>[6x]MIQGVIQKIAGPAVIAKGMLGARMYDICKVGEEGLVGEIIRLDGDTAFVQVYEDTSGLKVGEPVVSTGLPLAVELGPGMLNGIYDGIQRPLERIREKTGIYITRGVVVHALDREKKWAWTPMVKPGDEVRGGMVLGTVPEFGFTHKILVPPDVRGRVKEVKPAGEYTVEEPVVVLEDGTELKMYHTWPVRRARPVQRKLDPNTPFLTGMRILDVLFPVAMGGTAAIPGPFGSGKTVTQQSLAKWSNADVVVYVGCGERGNEMTDVLVEFPELTDPKTGGPLMHRTVLIANTSNMPVAAREASIYVGVTIAEYFRDQGFSVALMADSTSRWAEALREISSRLEEMPAEEGYPPYLAARLAAFYERAGKVITLGGEEGAVTIVGAVSPPGGDMSEPVTQSTLRIVGAFWRLDASLAFRRHFPAINWNGSYSLFTSALDPWYRENVAEDYPELRDAISELLQREAGLQEIVQLVGPDALQDAERLVIEVGRIIREDFLQQNAYHEVDAYCSMKKAYGIMKMILAFYKEAEAAIKRGVSIDEILQLPVLERIGRARYVSEEEFPAYFEEAMKEIQGAFKALA;>[6x]MDLLKKEYTGITYISGPLLFVENAKDLA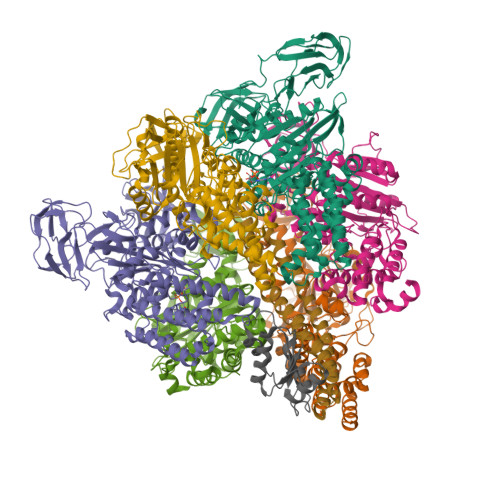YGAIVDIKDGTGRVRGGQVIEVSEEYAVIQVFEETTGLDLATTSVSLVEDVARLGVSKEMLGRRFNGIGKPIDGLPPITPEKRLPITGLPLNPVARRKPEQFIQTGISTIDVMNTLVRGQKLPIFSGSGLPANEIAAQIARQATVRPDLSGEGEKEEPFAVVFAAMGITQRELSYFIQEFERTGALSRSVLFLNKADDPTIERILTPRMALTVAEYLAFEHDYHVLVILTDMTNYCEALREIGAAREEIPGRRGYPGYMYTDLATIYERAGVVEGKKGSVTQIPILSMPDDDRTHPIPDLTGYITEGQIQLSRELHRKGIYPPIDPLPSLSRLMNNGVGKGKTREDHKQVSDQLYSAYANGVDIRKLVAIIGEDALTENDRRYLQFADAFERFFINQGQQNRSIEESLQIAWALLSMLPQGELKRISKDHIGKYYGQKLEEIWGAPQALD;>MSQVSPTRMNLLQRRGQLRLAQKGVDLLKKKRDALVAEFFGLVREAMEARKALDQAAKEAYAALLLAQAFDGPEVVAGAALGVPPLEGVEAEVENVWGSKVPRLKATFPDGALLSPVGTPAYTLEASRAFRRYAEALIRVANTETRLKKIGEEIKKTTRRVNALEQVVIPGIRAQIRFIQQVLEQREREDTFRLKRIKGKIEAREAEEEGGRPNPQVEIGAGL[2x];>[2x]MAVIADPETAQGFRLAGLEGYGASSAEEAQSLLETLVERGGYALVAVDEALLPDPERAVERLMRGRDLPVLLPIAGLKEAFQGHDVEGYMRELVRKTIGFDIKL>[2x]G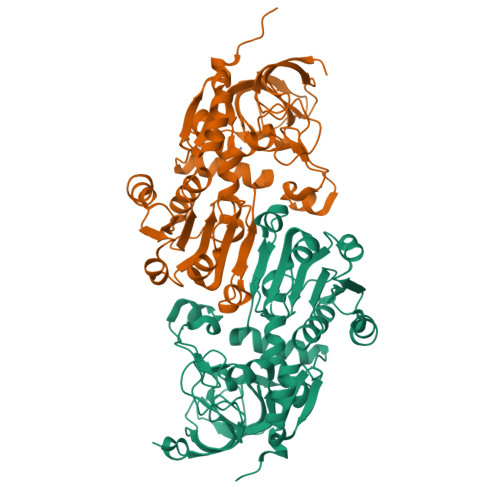PAAKSPENVYPVKTFGFAAKDSSGFFSPFNFSRRATGENDVQFKVLYCGTCNYDLEMSTNKFGMTKYPFVIGHEIVGVVTEIGSKVQKFKVGDKVGVGGFVGACEKCEMCVNGVENNCSKVESTDGHFGNNFGGCCNIMVVNEKYAVVWPENLPLHSGVPLLCAGITTYSPLRRYGLDKPGLNIGIAGLGGLGHLAIRFAKAFGAKVTLISSSVKKKREALEKFGVDSFLLNSNPEEMQGAYGTLDGIIDTMPVAHSIVPFLALLKPLGKLIILGVPEEPFEVPAPALLMGGKLIAGSAAGSMKETQEMIDFAAKHNIVADVEVIPIDYLNTAMERIKNSDVKYRFVIDVGNTLKSPSF> GASKGNLLSPDRILTVAHRGASGYVPEHTILSYETAQKMKADFIELDLQMTKDGKLIVMHDEKLDRTTNGMGWVKDHTLADIKKLDAGSWFNEAYPEKAKPQYVGLKVPTLEEVLDRFGKHANYYIETKSPDTYPGMEEKLIA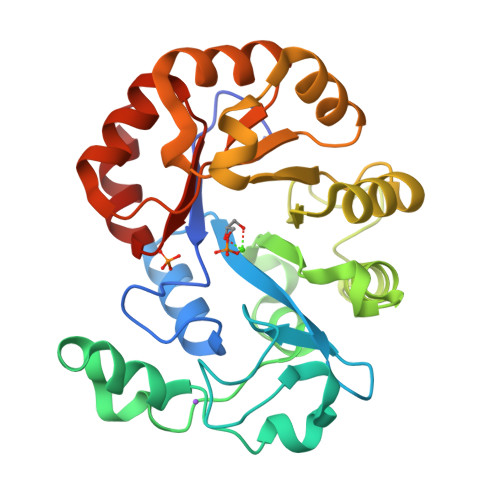SLQKHKLLGKHSKPGQVIIQSFSKESLVKVHQLQPNLPTVQLLEAKQMASMTDAALEEIKTYAVGAGPDYKALNQENVRMIRSHGLLLHPYTVNNEADMHRLLDWGVTGVFTNYPDLFHKVKKGY N-[2-({2-AMINO-6-ETHYL-5-[4-(3-METHOXYPROPYL)-2,2-DIMETHYL-3-OXO-3,4-DIHYDRO-2H-1,4-BENZOXAZIN-6-YL]PYRIMIDIN-4-YL}AMINO)ETHYL]NAPHTHALENE-2-SULFONAMIDE 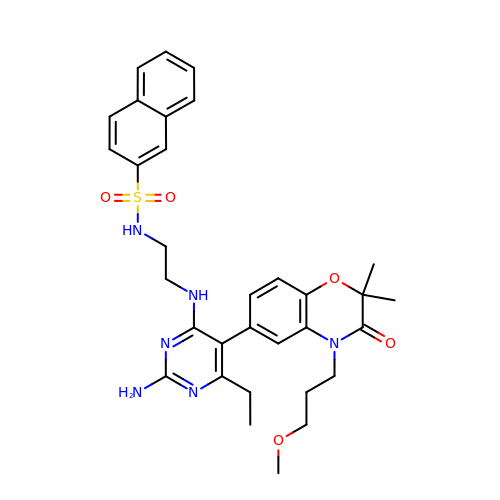| C32 H38 N6 O5 S | RRWBDAPAGFVYPT-UHFFFAOYSA-N> MFGLIGHLTSLEQARDVSRRMGYDEYADQGLEFWSSAPPQIVDEITVTSATGKVIHGRYIESCFLPEMLAARRFKTATRKVLNAMSHAQKHGIDISALGGFTSIIFENFDLASLRQVRDTTLEFERFTTGNTHTAYVICRQVEAAAKTLGIDITQATVAVVGATGDIGSAVCRWLDLKLGVGDLILTARNQERLDNLQAELGRGKILPLEAALPEADFIVWVASMPQGVVIDPATLKQPCVLIDGGYPKNLGSKVQGEGIYVLNGGVVEHCFDIDWQIMSAAEMARPERQMFASFAEAMLLEFEGWHTNFSWGRNQITIEKMEAIGEASVRHGFQPLALAI;> MRTPWDPPNPTFSLSSVSGDRRLMPQLEASLELDFQSESYKDAYSRINAIVIEGEQEAFDNYNRLAEMLPDQRDELHKLAKMEQRHMKGFMACGKNLSVTPDMGFAQKFFERLHENFKAAAAEGKVVTCLLIQSLIIECFAIAAYNIYIPVADAFARKITEGVVRDEYLHRNFGEEWLKANFDASKAELEEANRQNLPLVWLMLNEVADDARELGMERESLVEDFMIAYGEALENIGFTTREIMRMSAYGLAAV

The earlier discovery of the pathway responsible for alkane biosynthesis in cyanobacteria allowed the conversion from solar energy to alkanes through photosynthesis, without providing external carbon sources. This two-step pathway utilizes two water-soluble enzymes, namely acyl-acyl carrier protein (acyl-ACP) reductase (AAR) and aldehyde-deformylating oxygenase (ADO). AAR catalyzes the first step of this pathway, reducing the substrate fatty acyl-ACP/fatty acyl-coenzyme A (acyl-CoA) into the corresponding aldehyde in a NADPH-dependent manner. Subsequently, ADO catalyzes the conversion of fatty aldehyde into alk(a/e)ne with one carbon shorter (Cn-1 hydrocarbon) and the formate as a C1-derived form. Here we report the crystal structure of AAR from Synechococcus elongatus PCC 7942 (SeAAR) in its apo form (AARapo), together with three structures of AAR in complex with ADO from the same species of cyanobacteria (SeADO), in which AAR binds either substrate or substrate/cofactor.

We obtained the AARstearoyl-CoA–ADO structure using the AAR C294S mutant, which avoid spontaneous formation of the acyl-enzyme intermediate, and solved the structure at 3.01 Å resolution. In this structure, the entire stearoyl-CoA molecule occupies the long L-shaped channel of AAR. The CoA moiety occupies the same cleft in which NADPH was observed to bind in the AARNADPH–ADO structure. The main cause of this shift is that the C294S mutant is not able to form a thioester bond, and thus fails to fix the stearic chain at the active site of AAR. This extended conformation of stearoyl-CoA induces movement of the Fr-I region of AAR. Thus, Y23 and Y26, which form the terminal end of the acyl-tunnel in the AARthioester–ADO structure, are distant from the stearic moiety in the AARstearoyl-CoA–ADO structure. These changes result in a wider opening at the surface of the AAR molecule. Furthermore, M21, Y23, and Y26 of AAR form additional hydrogen bonds with R218 and M221 from helix 8 of ADO, and the conformation of M221 of ADO alters so that it no longer seals the acyl-tunnel of AAR as it does in the AARthioester–ADO structure. Together, these structural changes facilitate the release of produced aldehydes from AAR, suggesting that the AARstearoyl-CoA–ADO structure mimics the aldehyde-releasing state of AAR, in which the free aldehyde is released, ready to be transferred to ADO.>GPLGSLVNVIRRESGNPDLLELLMDLNCYTLEVTEGYLKKVNVTEVNGDNVLGPIHVITTVVSSLVRNGLLIQSSKFISKVLLTVESIVMSLPKDETMLGGIFWLSNLSRLPAFAANQKTLYEANGGDEKDKLTLIYLNDLENETLKVFDKIYSTWLVKFMKHASAHIEIFDMVLNEKLFKNSGDEKFAKLFTFLNEFDAVLCKFQVVDSMHTKIFNDTLKYLNVMLFNDLITKCPALNWKYGYEVDRNIERLVSWFEPRIEDVRPNLIQIIQAVKILQLKISNLNEFKLLFDFWYALNPAQIQAILLKYKPANKG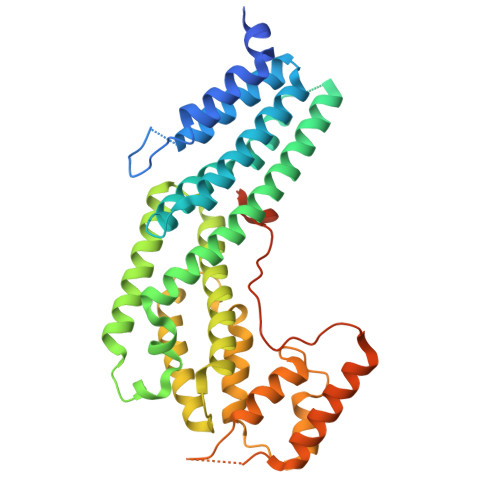EAGVPNEILNYLANVIKRENLSLPGKMEIMLSAQFDSAKNHLRYDTSAITQNSNTEGLATVSKIIKLDRK[2x]> MGSSHHHHHHSSPISPIETVPVKLKPGMDGPKVKQWPLTEEKIKALVEICTEMEKEGKISKIGPENPYNTPVFAIKKKDSTKWRKLVDFRELNKRTQDFWEVQLGIPHPAGLKKKKSVTVLDVGDAYFSVPLDEDFRKYTAFTIPSINNETPGIRYQYNVLPQGWKGSPAIFQSSMTKILEPFRKQNPDIVIYQYMDDLYVGSDLEIGQHRTKIEE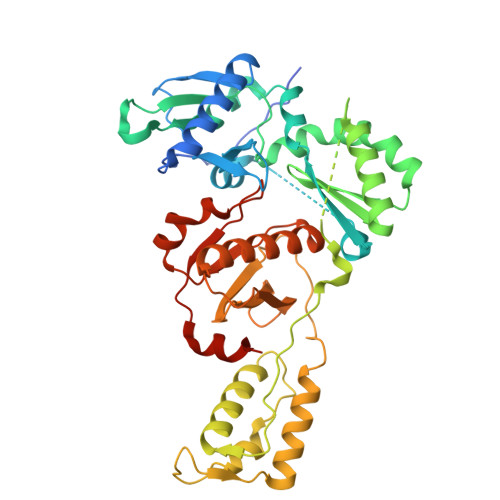LRQHLLRWGLTTPDKKHQKEPPFLWMGYELHPDKWTVQPIVLPEKDSWTVNDIQKLVGKLNWASQIYPGIKVRQLSKLLRGTKALTEVIPLTEEAELELAENREILKEPVHGVYYDPSKDLIAEIQKQGQGQWTYQIYQEPFKNLKTGKYARMRGAHTNDVKQLTEAVQKITTESIVIWGKTPKFKLPIQKETWETWWTEYWQATWIPEWEFVNTPPLVKLWYQLEKEPIVGAETF> PRTQFSGLRRELPPSVRLLTLARWGPETLLLRLEHQFAVGEDSGRNLSSPVTLDLTNLFSAFTITNLRETTLAANQLLAYASRLQWTT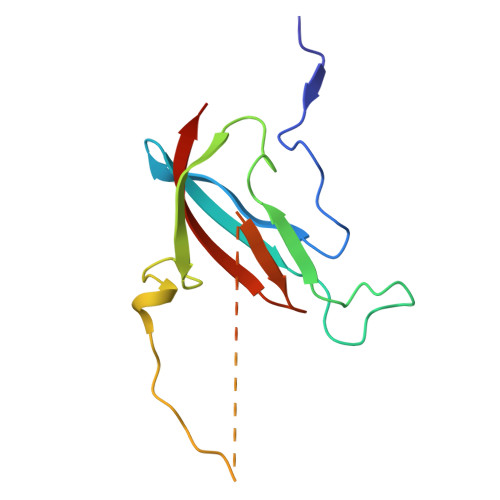DTGPTPHPSPSRPVSATITLQPMEIRTFLASVQWEEDG> MDYKDDDDKMSAKKI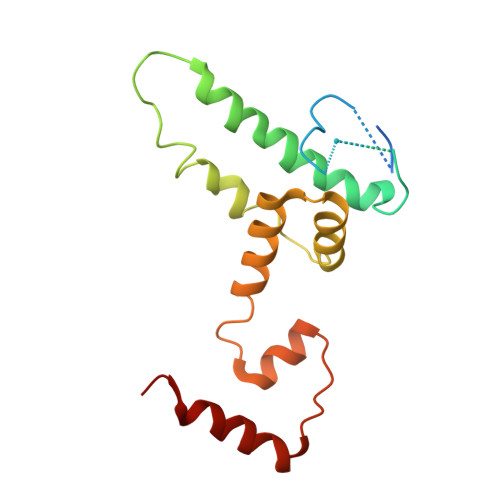VLKSSDGESFEVEEAVALESQTIAHMVEDDCVDNGVPLPNVTSKILAKVIEYCKRHVEAAASKAEAVEGAATSDDDLKAWDADFMKIDQATLFELILAANYLNIKNLLDLTCQTVADMIKGKTPEEIRTTFNIKNDFTPEEEEEVRRENQWAFE>LPDLKIEKLEEGVFVHTSFEEVNGWGVVTKHGLVVLVNTDAYLIDTPFTATDTEKLVNWFVERGYEIKGTISSHFHSDSTGGIEWLNSQSIPTYASELTNELLKKSGKVQAKYSFSEVSYWLVKNKIEVFYPGPGHTQDNLVVWLPESKILFGGCFIK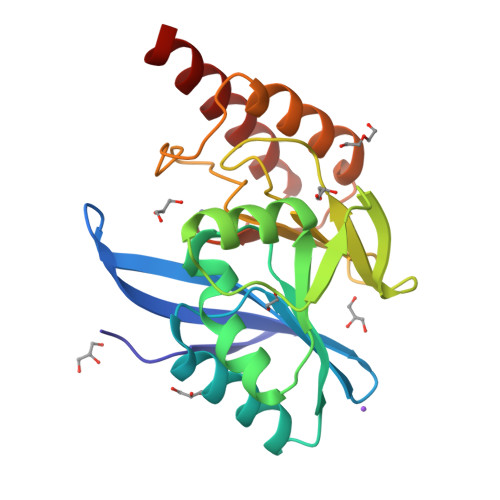PHGLGNLGDANLEAWPKSAKILMSKYGKAKLVVSSHSEKGDASLMKRTWEQALKGLKESK[2x]> SHHHHHHAGAGSHCQKTSLRVNFEDIGWDSWIIAPKEYEAYECKGGCFFPLADDVTPTKHAIVQTLVHLKFPTKVGKACCV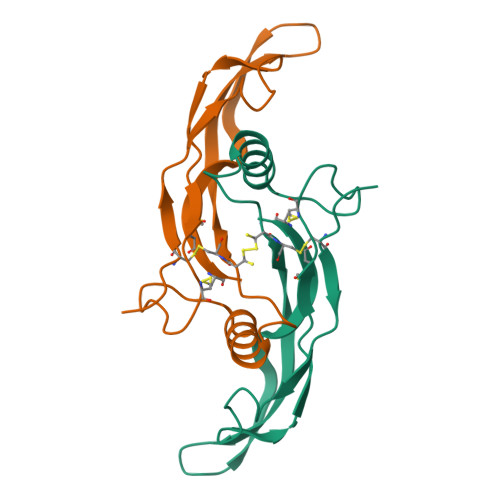PTKLSPISVLYKDDMGVPTLKYHYEGMSVAECGCR> LPTHLYKNFTVQELALKLKGKNQEFCLTAFMSGRSLVRACLSDAGHEHDTWFDTMLGFAISAYALKSRIALTVEDSPYPGTPGDLL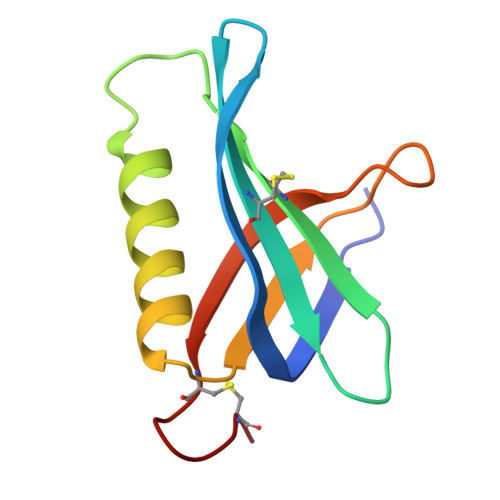ELQICPLNGYCE> HMIALLAPGQGSQTEGMLSPWLQLPGAADQIAAWSKAADLDLARLGTTASTEEITDTAVAQPLIVAATLLAHQELARRCVLAGKDVIVAGHSVGEIAAYAIAGVIAADDAVALAATRGAEMAKACATEPTGMSAVLGGDETEVLSRLEQLDLVPANRNAAGQIVAAGRLTALEKLAEDPPAKARVRALGVAGAFHTEFMAPALDG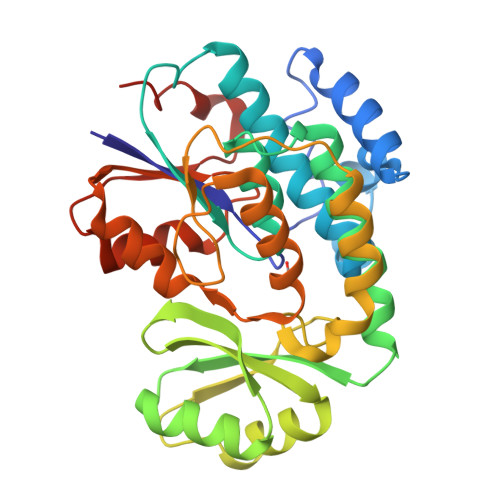FAAAAANIATADPTATLLSNRDGKPVTSAAAAMDTLVSQLTQPVRWDLCTATLREHTVTAIVEFPPAGTLSGIAKRELRGVPARAVKSPADLDELANL To further explore this issue, we have conducted biochemical and crystallographic studies on the interactions of six GSTOs from T. versicolor with chemical libraries. The six TvGSTOs (named TvGSTO1S to TvGSTO6S) used in this study are representatives of the twelve TvGSTOs that have a catalytic serine, while four others have a cysteine instead. In this study, we demonstrated at the biochemical and structural level that T. versicolor GSTs that belong to the Omega class interact with polyphenolic compounds found in wood, and in particular with flavonoids such as dihydrowogonin and naringenin. The ability of TvGSTOs to bind polyphenols through different sites suggests that fungal GSTs could be involved in the transport of various polyphenols.

In order to get a detailed picture of the ligand binding sites of TvGSTO3S, we determined the structures of several complexes with free GSH, or some glutathionylated derivatives GS-R (glutathionyl-dinitrobenzene GS-DNB and glutathionyl-phenylacetophenone GS-PAP), or some of the HBPs identified by TSA (2,4-, 3,4-, 2,3,4-, 2,4,4′- HBPs). TvGSTO3S harbors a canonical GSH binding site (G-site) made up of polar residues from the N-terminal domain which stabilizes the glutathionyl moiety (GS-) of the tested ligands. On the contrary, the hydrophobic binding site (H-site) which hosts the -R group of the GS-R ligand has a singular shape relative to most GSTs. The crystal structures of the different complexes show that this pocket is perfectly suited to accommodate polyaromatic ligands, due to its strong hydrophobic character, while two polar residues are found at the entrance close to the G-site. The phenylacetophenone group of GS-PAP fully fills the cavity, on the contrary to the more polar -R group of GS-DNB that does not enter it and is only slightly stabilized at its entrance, at the interface with the G-site.

>MSSTKQITLYTATFSPYAHRVRIALEEAGAEYTTYDVDILRNMPDWFPLVNPLKKIPAMTFGGPEVPPDQPSPESAKIAESLAMLEFIADLFPDAKLLPTDPVLRARARTFMALYENYVNGQFRDVWFLGTPADPLLQALEMLQGALPPDGGFAAGEWSIADAAVIPFLARMFPYLEAGLGLYSKEDGVKMRKAMASERFARIRQYVRDCRARPSFANTWAGDAEQVEAAKTVPMLRVGEHHHHHH[2x]> MSSPLKNALVTAMLAGGALSSPTKQHVGIPVNASPEVGPGKYSFKQVRNPNYKFNGPLSVKKTYLKYGVPIPAW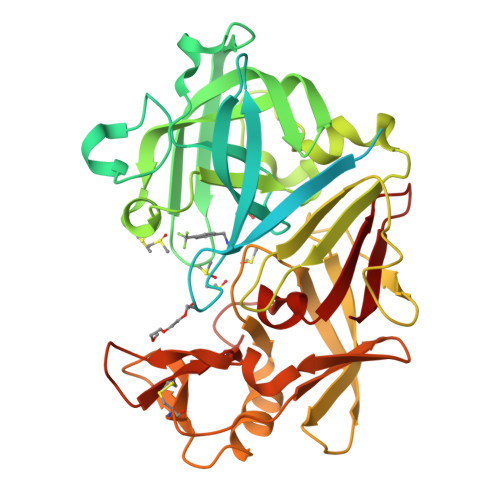LEDAVQNSTSGLAERSTGSATTTPIDSLDDAYITPVQIGTPAQTLNLDFDTGSSDLWVFSSETTASEVDGQTIYTPSKSTTAKLLSGATWSISYGDGSSSSGDVYTDTVSVGGLTVTGQAVESAKKVSSSFTEDSTIDGLLGLAFSTLNTVSPTQQKTFFDNAKASLDSPVFTADLGYHAPGTYNFGFIDTTAYTGSITYTAVSTKQGFWEWTSTGYAVGSGTFKSTSIDGIADTGTTLLYLPATVVSAYWAQVSGAKSSSSVGGYVFPCSATLPSFTFGVGSARIVIPGDYIDFGPISTGSSSCFGGIQSSAGIGINIFGDVALKAAFVVFNGATTPTLGFASK> MGEKQEEEGEEEKEGKGEGGGEGGREEEDEDGSAPVVSWLRIVEERECHEETDEAPETKIALPFSAQRSSRGFEARQVEVL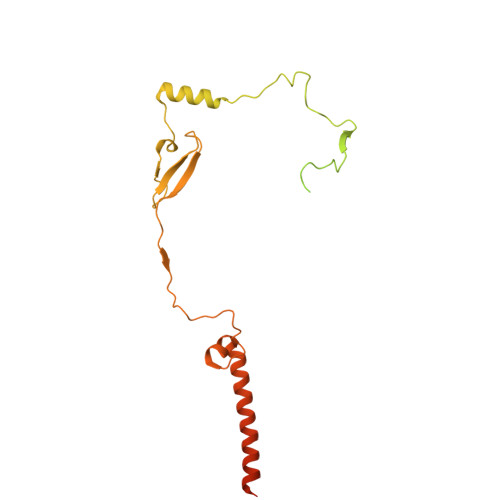VSANSAFLLSVLLASLFLSSSLPSFCPPRFLLSVLLALFKDKMAGDAPAAAAAPQQAGRTASASGVRTPGYLDLVGHSLKATSMDHGMQYSSIYWETSHRTYLPFWASLTQKFSWKIMDDQIRSFLRLPKPVTTEPFVFSSGSPYIRRYFGDADISVPVPLHAPAHFAFVPTGTVSPWEETGMETGPQGAAARGAAATAFRAVLESAWKCDIDEQIKEKLHSRAGAGAFHASGSTGGCPIPTDF>[2x]MLAKRIDAALIVKDGRVVEGSNFENLRDSGDPVELGKFYSEIGIDELSFWDITASVEKRKTMLELVEKVAEQIDIPFTVGGGIHDFETASELILRGADKVEINTAAVENPSLI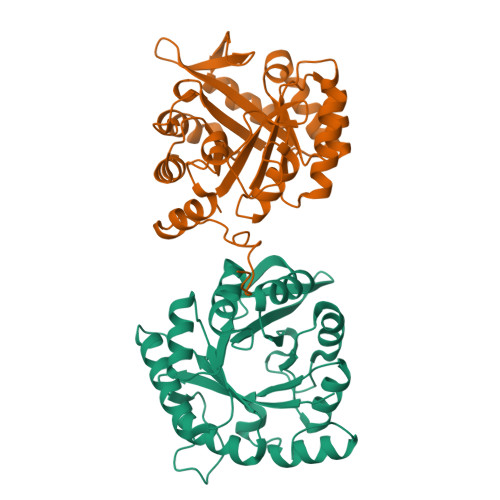TQIAQTFGSQAVVVYIAAKRVDGEFMVFTYSGTKNTGILLRDWVVEVEKRGAGEIVLGSIDRLGTKSGYDTEMIRFVRPLTTLPIIAHRGAGKMEHFLEAFLAGADAAKADSVFHFREIDVRELKEYLKKHGVNVRLEGLGSLEHHHHHH>MSQISKTHSRLAGRNAKPFDLKNITNDAVASLSRIGLVFDHAVVQDQIKALAKAGAFRSGSAMDSNFTAPVTTPSIPTPIQFLQTWLPGFVKVMTAARKIDEIIGIDTVGSWEDQEIVQGIVEPAGTAVEYGDHTNIPLTSWNANFERRTIVRGELGMMVGTLEEGRASAIRLNSAETKRQQAAIGLEIFRNAIGFYGWQSGLGNRTYGFLNDPNLPAFQTPPSQGWSTADWAGIIGDIREAVRQLRIQSQDQIDPKAEKITLALATSKVDYLSVTTPYGISVSDWIEQTYPKMRIVSAPELSGVQMKAQEPEDALVLFVEDVNAAVDGSTDGGSVFSQLVQSKFITLGVEKRAKSYVEDFSNGTAGALCKRPWAVVRYLGI[11x];>[5x]MAKSKRKIDENGYMTIEGCPISSYGVFQYSAGQLGLPGDPMRIVNVYRPESAVSDPEYIESLKNLPLIDEHEMLSGFDDDDDSVAPEDKGVEGIITSNAYYEAPWARGDIRIYSRNMQNQLERGKEDLSLGYSCRYTEQPGIWNGTPYEVV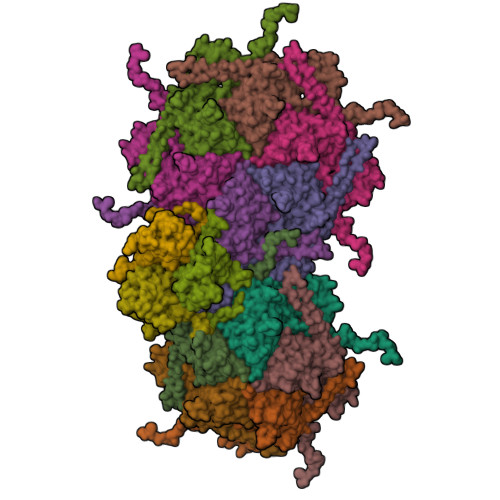QDKMRGNHIALVKEGRVPGARVLDGLCFDHLSFDFRPSDEGNEMSLKKAKQKPPVQRVGQAADSAVEELRALWPKLSASVQKFLGEEAQEPEHQEGAAAPAEPTDSEHMTEHPTLEGAQKDNEEHEEAPSVVDPAVAAAESERQESAASEMSGEGEVAELISQVKAILARLEGTAAEGADEEHGEGKDVVEGLEEQSSLSGSQTASDDGGEGKDNSEELPEMAQKNAQDAAIRGLYRDIAAKDRLYKRLSSVVGAFDHRAMDSAEVAVYGVKKLNINCAKGQEALALDMYLKGVEASRGAASRQSKAQDSAGSAPQCAELDSYLKGE;>MFQKQVYRQYTPGFPGDLIEDGPKRARPGRIMSLSAVNPAATATGPNRISRAFGYAGDVSALGEGQPKTIAARASEVVIGGANFFGVLGHPKHYALFGSAGDSLAPSYDLPDGAEGEFFDMATGLVVEIFNGAATALDLDYGDLVAYVPNNLPTADNALGLPAGALVGFKAGSMPTGLVQIPNARIVNAISLPAQSAGNLVAGVTIVQLTQ[3x]> GPAKQYDSVECPFCDEVSKYEKLAKIGQGTFGEVFKARHRKTGQKVALKKVLMENEKEGFPITALREIKILQLLKHENVVNLIEICRTKASPYNRCKGSIYLVFDFCEHDLAGLLSNVLVKFTLSEIKRVMQMLLNGLYYIHRNKILHRDMKAANVLITRDGVLKLADFGLARAFSLAKNSQP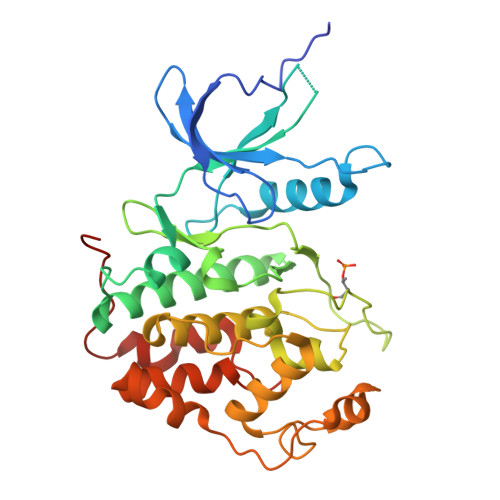NRYTNRVVTLWYRPPELLLGERDYGPPIDLWGAGCIMAEMWTRSPIMQGNTEQHQLALISQLCGSITPEVWPNVDNYELYEKLELVKGQKRKVKDRLKAYVRDPYALDLIDKLLVLDPAQRIDSDDALNHDFFWSDPMPSDLKGMLST Carbonic anhydrase (CA; EC 4.2.1.1) is a zinc containing enzyme which catalyzes a reversible reaction to form bicarbonate from carbon dioxide and water. The budding yeast Saccharomyces cerevisiae encodes a single copy of CA, termed Nce103 after the non-classical export pathway where it was identified for the first time. Nce103 is an efficient β-CA who shows high CO2 hydrase activity, with a kcat of 9.4 × 105 s-1 and kcat/Km of 9.8 × 107 M-1 s-1. Nce103 contains all conserved residues of the active site in the plant type β-CAs, and a relatively divergent N-terminal region.

Thus, we constructed the truncated version Nce103ΔN13 which enabled us to determine its crystal structure at 2.04 Å resolution. The overall structure of Nce103 contains two molecules in an asymmetric unit. The missing electron density of the N-terminal 6× His-tag, residues His14-Ser16 and Pro41-Gln48 of each subunit indicates their high degree of flexibility. The N-terminal arm is composed of two α-helices that extend away from the rest of the molecule, making extensive contacts with the other molecule in the asymmetric unit. Two subunits form a very tight homodimer with a buried interface of 3,027 Å2, bringing the two zinc binding pockets close to each other. Each subunit contains a zinc ion that resides at the interface between two subunits, with three coordinating residues (Cys57, Cys115 and His112) from the same subunit, and a water molecule Wat263A/Wat260B as the fourth to complete the tetrahedral coordination. In the substrate binding pocket, there is a flat trilobed piece of density, reminiscent of an acetate molecule, which is an analog of the substrate bicarbonate. Compared to that in PSCA (or Can2), the acetate molecule (ACT) in Nce103 is far away from the zinc ion (3.53 vs 2.65 Å). The two tunnels in the homodimer point to the opposite directions towards the surface. It is worth noting that this tunnel is funnel-shaped, widely open toward the solvent but has a narrow gorge (cross section radius ~2.1 Å) in the vicinity of the acetate ion, suggesting that the linear CO2 (with a length of ~3.3 Å) molecule can freely diffuse toward the active sites, consistent with the diffusion-control catalytic mechanism of β-CAs. Nce103ΔN13 shows almost the same activity as the full length Nce103, whereas the activity of Nce103ΔN50 has been completely abolished.

>MHHHHHHGHNSNLQDILAANAKWASQMNNIQPTLFPDHNAKGQSPHTLFIGCSDSRYNENCLGVLPGEVFTWKNVANICHSEDLTLKATLEFAIICLKVNKVIICGHTDCGGIKTCLTNQREALPKVNCSHLYKYLDDIDTMYHEESQNLIHLKTQREKSHYLSHCNVKRQFNRIIENPTVQTAVQNGELQVYGLLYNVEDGLLQTVSTYTKVTPK[2x]>[2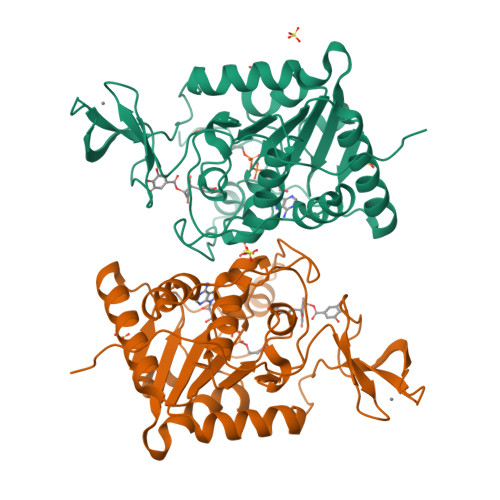x]GIDPFTADKGKCGLPEIFDPPEELERKVWELARLVWQSSSVVFHTGAGISTASGIPDFRGPHGVWTMEERGLAPKFDTTFESARPTQTHMALVQLERVGLLRFLVSQNVDGLHVRSGFPRDKLAELHGNMFVEECAKCKTQYVRDTVVGTMGLKATGRLCTVAKARGLRACRGELRDTILDWEDSLPDRDLALADEASRNADLSITLGTSLQIRPSGNLPLATKRRGGRLVIVNLQPTKHDRHADLRIHGYVDEVMTRLMKHLGLEIPAWDGPRVLERALPPLPRPPTPKLEPKEESPTRIN> GPSPEIGQIVKIVKGRDRDQFSVIIKRVD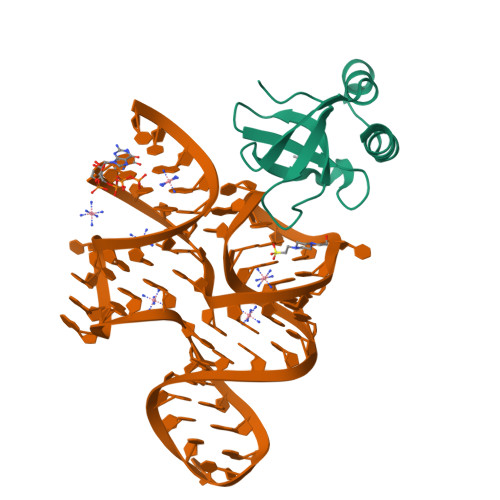DRFVYIADGDKRKVDRAKRKNMNHLKLIDHISPEVRHSFEETGKVTNGKLRFALKKFLEEHADLLKEGE> SNAMRNKNMSTIYQTSATASAGRNGVVSTEDKLLELNLSYPKEMGGSGTATNPEQLFAVGYAACFSNAILHVAREAKV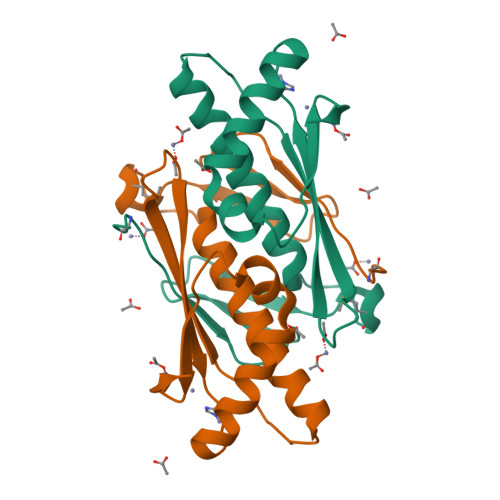ALKEAPVTATVGIGPNGQGGFALSVALAAHIALEDEQARQLVTVAHQVCPYSNAVRGNIDVQVSVNGLAL> MHHHHHHTTSVDPTSGPQASGTEQNRSSLDTAAARKLATTTKTVPQMQ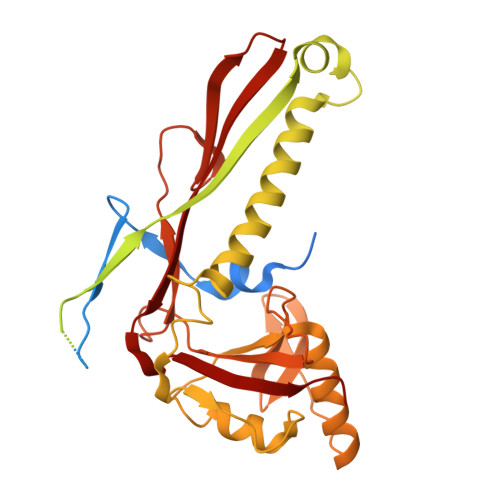GISSRWLLRVLPWTQVNGGTYRVNRRLTHTLGDGQVEFVNTGAEVRVIPEELRELAPLRGFTDTPTLEALAGRFAQHEFAPGDVLAQQDQPADRIILIAHGKLDRLGTGKYGGETVQGQLAGGDHLGAAALLDGGAAWEHTVRAVTRVTALTLSRGDYEQVLGGSESLRAHVEAFRAALVPAQNKHGEAAIEVAAGHVGEPSLPGTFADYDLAPREYELSVAQTVLKIHSRVADLYNDPMNQMDQQLRLTVEALRERQEHEMINNREFGLLHNADLKQRIHTRSGPPTPDDLDELISRRRKTQVLLAHPRTIAAIGREWNARGIYPTGAELHGTDVRAWRGIPLLPCNKIPVTPEQTSSIIAMRLGEENQGVVGLHQTGIPDEYQPGLSVRFMGINDQAVIQYLVSAYYSAAVLVPDALGILEDVEIGH>MSSQVEHPAGGYKKLFETVEELSSPLTAHVTGRIPLWLTGSLLRCGPGLFE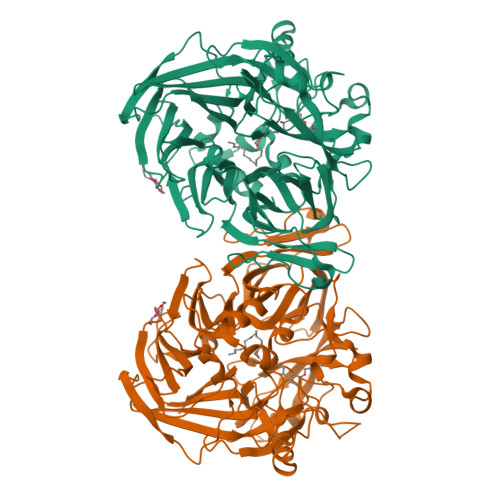VGSEPFYHLFDGQALLHKFDFKEGHVTYHRRFIRTDAYVRAMTEKRIVITEFGTCAFPDPCKNIFSRFFSYFRGVEVTDNALVNIYPVGEDYYACTETNFITKVNPETLETIKQVDLCNYVSVNGATAHPHIENDGTVYNIGNCFGKNFSIAYNIVKIPPLQADKEDPISKSEIVVQFPCSDRFKPSYVHSFGLTPNYIVFVETPVKINLFKFLSSWSLWGANYMDCFESNETMGVWLHIADKKRKKYINNKYRTSPFNLFHHINTYEDHEFLIVDLCCWKGFEFVYNYLYLANLRENWEEVKKNARKAPQPEVRRYVLPLNIDKADTGKNLVTLPNTTATAILCSDETIWLEPEVLFSGPRQAFEFPQINYQKYGGKPYTYAYGLGLNHFVPDRLCKLNVKTKETWVWQEPDSYPSEPIFVSHPDALEEDDGVVLSVVVSPGAGQKPAYLLILNAKDLSEVARAEVEINIPVTFHGLFKKS[2x]>[2x]AECSVDIQGNDQMQFNTNAITVDKSCKQFTVNLSHPGNLPKNVMGHNWVLSTAADMQGVVTDGMASGLDKDYLKPDDSRVIAHTKLIGSGEKDSVTFDVSKLKEGEQYMFFCAAAAH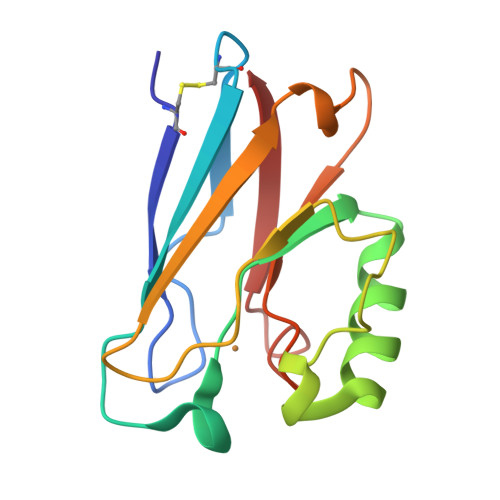AAAAMKGTLTLK3-[5-[(4~{a}~{R},8~{a}~{S})-4-oxidanylidene-3-propan-2-yl-4~{a},5,8,8~{a}-tetrahydrophthalazin-1-yl]-2-methoxy-phenyl]-~{N}-(3-methoxyphenyl)prop-2-ynamide 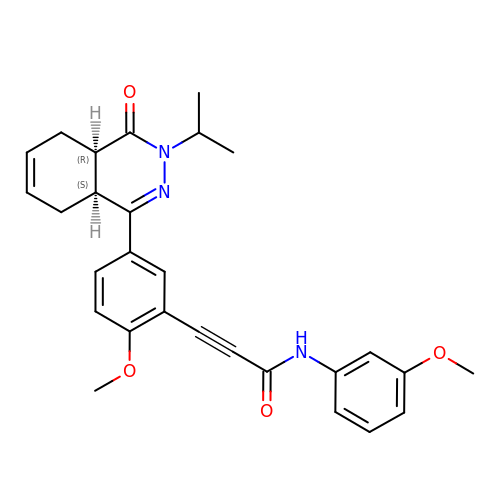| C28 H29 N3 O4 | FLXJAXHKQHLPKX-BJKOFHAPSA-N> MGSSHHHHHHSAGENLYFQGTLPRETDEEPEEPGRRGSFVEMVDNLRGKSGQGYYVEMTVGSPPQTLNILVDTGSSNFAVGAAPHPFLHRYYQRQLSSTYRDLRKGVYVPYTQGKWEGELGTDLVSIPHGPNVTVRANIAAITESDKFFINGSNWEGILGLAYAEIARPDDSLEPFFDSLVKQTHVPNLFSLQLCGAGFPLNQSEVLASVGGSMIIGGIDHSLYTGSLWYTPIRREWYYEVIIVRVEINGQDLKMDCKEYNYDKSIVDSGTTNLRLPKKVFEAAVKSIKAASSTEKFPDGFWLGEQLVCWQAGTTPWNIFPVISLYLMGEVTNQSFRITILPQQYLRPVEDVATSQDDCYKFAISQSSTGTVMGAVIMEGFYVVFDRARKRIGFAVSA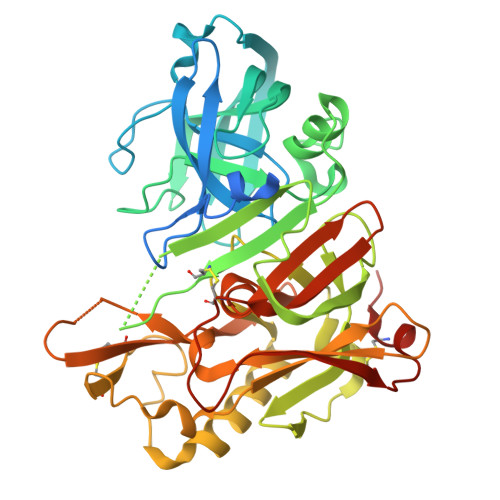CHVHDEFRTAAVEGPFVTLDMEDCGYNIPQTDEST> GSMADEATRRVVSEIPVLKTNAGPRDRELWVQRLKEEYQSLIRYVENNKNADNDWFRLESNKEGTRWFGKCWYIHDLLKYEFDIEFDIPITYPTT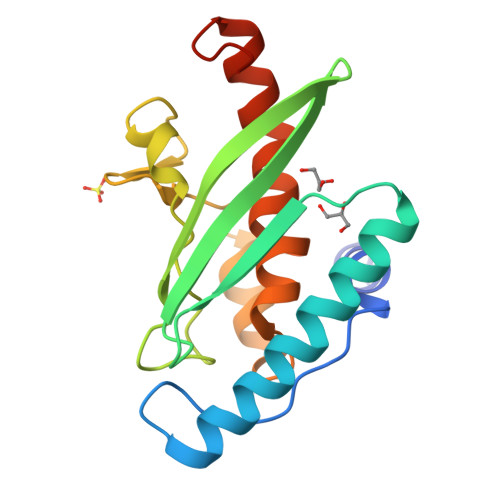APEIAVPELDGKIAKMYRGGKIELTDHFKPLWARNVPKFGLAHLMALGLGPWLAVEIPDLIQKGVIHHKEKCNQ>[2x]MAAATGGLTPEQIIAVDGAHLWHPYSSIGREAVSPVVAVAAHGAWLTLIRDGQPIEVLDAMSSWWTAIHGHGHPALDQALTTQLRVMNHVMFGGLTHEPAARLAKLLVDIT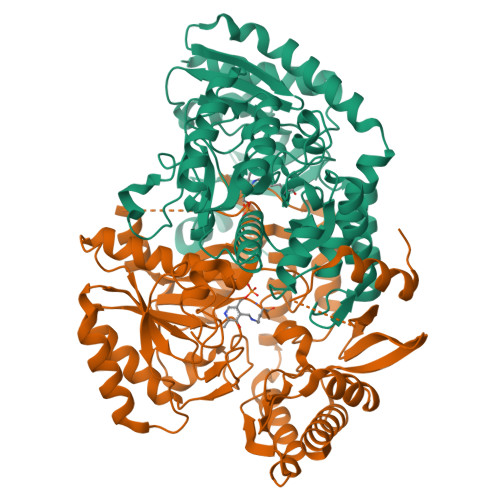PAGLDTVFFSDSGSVSVEVAAKMALQYWRGRGLPGKRRLMTWRGGYHGDTFLAMSICDPHGGMHSLWTDVLAAQVFAPQVPRDYDPAYSAAFEAQLAQHAGELAAVVVEPVVQGAGGMRFHDPRYLHDLRDICRRYEVLLIFDEIATGFGRTGALFAADHAGVSPDIMCVGKALTGGYLSLAATLCTADVAHTISAGAAGALMRGPTFMANPLACAVSVASVELLLGQDWRTRITELAAGLTAGLDTARALPAVTDVRVCGAIGVIECDRPVDLAVATPAALDRGVWLRPFRNLVYAMPPYICTPAEITQITSAMVEVARLVGSLP>[2x]MGSDKIHHHHHHMVVNLEGKISKIGQNMKSSIIREILKFAADKDAISFGGGVPDPETFPRKELAEIAKEIIEKEYHYTLQYSTT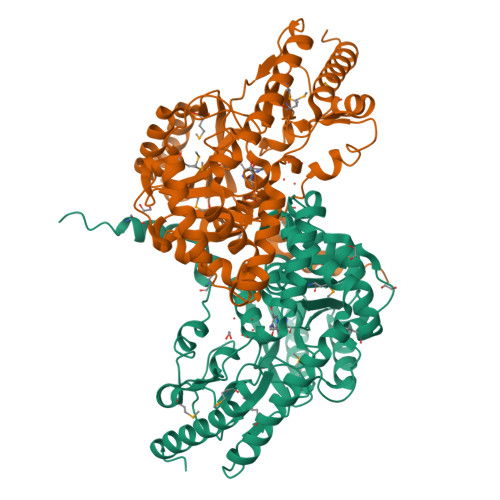EGDPVLKQQILKLLERMYGITGLDEDNLIFTVGSQQALDLIGKLFLDDESYCVLDDPAYLGAINAFRQYLANFVVVPLEDDGMDLNVLERKLSEFDKNGKIKQVKFIYVVSNFHNPAGVTTSLEKRKALVEIAEKYDLFIVEDDPYGALRYEGETVDPIFKIGGPERVVLLNTFSKVLAPGLRIGMVAGSKEFIRKIVQAKQSADLCSPAITHRLAARYLERYDLLEQLKPTIELYRRKRTVMLNALEEYFSDIPGVKWVKSEGGLFIWLTLPEGFDTWEMFEYAKRKKVFYVPGRVFKVYDEPSPSMRLSFCLPPDEKIVEGIKRLREVVLEYGKEKHLL>MTAASLDPTAFSLDAASLAARLDAVFDQALRERRLVGAVAIVARHGEILYRRAQGLADREAGRPMREDTLFRLASVTKPIVALAVLRLVARGELALDAPVTRWLPEFRPRLADGSEPLVTIHHLLTHTSGLGYWLLEGAGSVYDRLGISDGIDLRDFDLDENLRRLASAPLSFAPGSGWQYSLALDVLGAVVERATGQPLAAAVDALVAQPLGMRDCGFVSAEPERFAVPYHDGQPEPVRMRDGIEVPLPEGHGAAVRFAPSRVFEPGAYPSGGAGMYGSADDVLRALEAIRANPGFLPETLADAA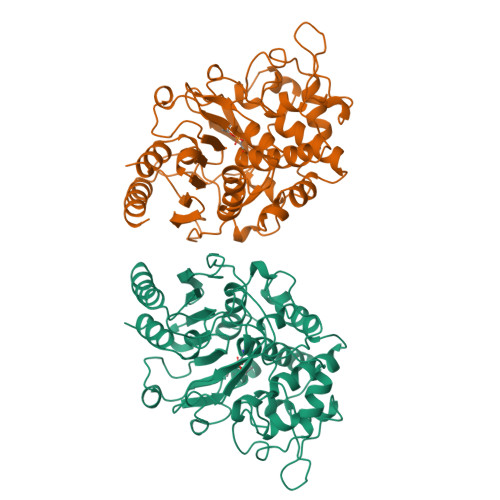RRDQAGVGAETRGPGWGFGYLSAVLDDPAAAGTPQHAGTLQWGGVYGHSWFVDRALGLSVLLLTNTAYEGMSGPLTIALRDAVYAR[2x]>MVIALVTHARHFAGPAAVEALTQDGYTVVCHDASFADAAERQRFESENPGTIALAEQKPERLVDATLQHGEAIDTIVSNDYIPRPMNRLPLEGTSEADIRQMFEALSIFPILLLQSAIAPLRAAGGASVIFITSSVGKKPLAYNPLYGPARAATVALVESAAKTLSRDGILLYAIG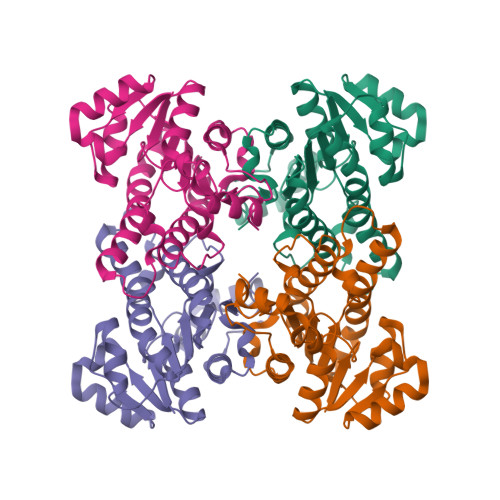PNFFNNPTYFPTSDWENNPELRERVDRDVPLGRLGRPDEMGALITFLASRRAAPIVGQFFAFTGGYLP[8x]>GMKNNNVTEKELFYILDLFEHMKVTYWLDGGWGVDVLTGKQQREHRDIDIDFDAQHTQKVIQKLEDIGYKIEVHWMPSRMELKHEEYGYLDIHPINLNDDGSITQANPEGGNYVFQNDWFSETNYKDRKIPCISKEAQLLFHSGYDLTE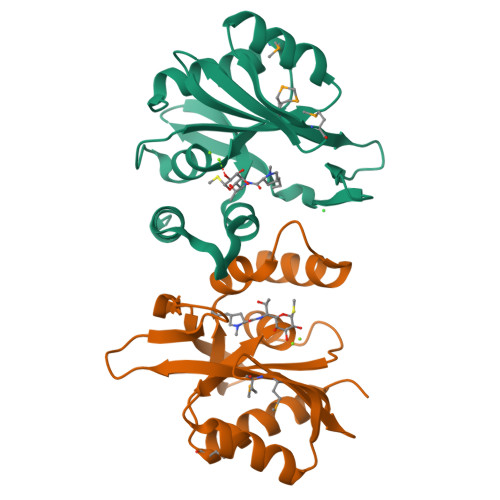TDHFDIKNLKSIT[2x]>[2x]MTDTIFDYVIVGGGTAGSVLANRLSARPENRVLLIEAGIDTPENNIPPEIHDGLRPWLPRLSGDKFFWPN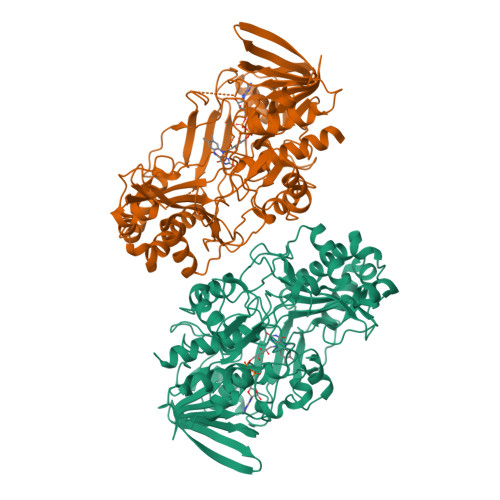LTIHRAAEHPGITREPQFYEQGRLLGGGSSVNMVVSNRGLPRDYDEWQALGADGWDWQGVLPYFIKTERDADYGDDPLHGNAGPIPIGRVDSRHWSDFTVAATQALEAAGLPNIHDQNARFDDGYFPPAFTLKGEERFSAARGYLDASVRVRPNLSLWTESRVLKLLTTGNAITGVSVLRGRETLQVQAREVILTAGALQSPAILLRTGIGPAADLHALGIPVLADRPGVGRNLWEHSSIGVVAPLTEQARADASTGKAGSRHQLGIRASSGVDPATPSDLFLHIGADPVSGLASAVFWVNKPSSTGWLKLKDADPFSYPDVDFNLLSDPRDLGRLKAGLRLITHYFAAPSLAKYGLALALSRFAAPQPGGPLLNDLLQDEAALERYLRTNVGGTWHASGTARIGRADDSQAVVDKAGRVYGVTGLRVADASIMPTVPTANTNLPTLMLAEKIADAILTQA N-(beta-L-Fucopyranosyl)-biphenyl-3-carboxamide 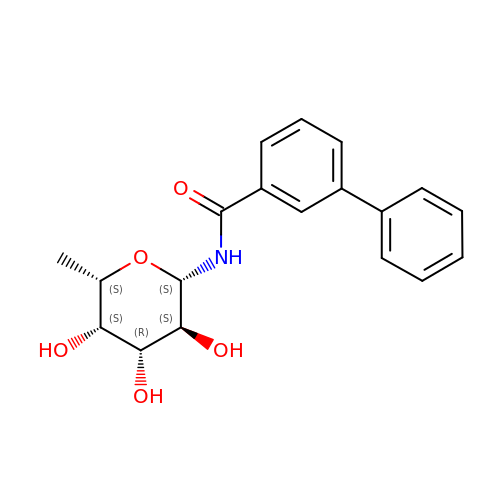| C19 H21 N O5 | KFRIUGARMXQWFO-QFFBLRJASA-N> ITGRPEWIWLALGTALMGLGTLYFLVKGMGVSDPDAKKFYAITTLVPAIAFTMYLSMLLGYGLTMVPF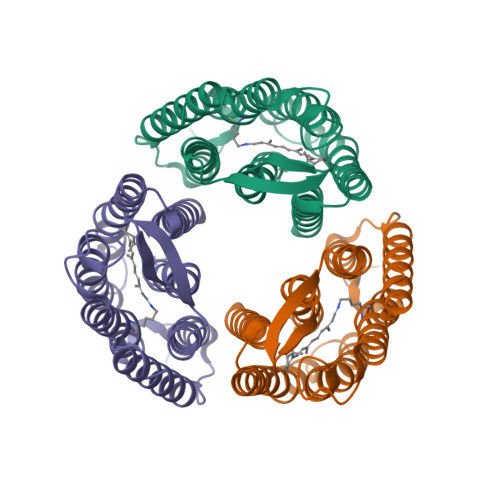GGEQNPIYWARYADWLFTTPLLLLDLALLVDADQGTILALVGADGIMIGTGLVGALTKVYSYRFVWWAISTAAMLYILYVLFFGFTSKAESMRPEVASTFKVLRNVTVVLWSAYPVVWLIGSEGAGIVPLNIETLLFMVLDVSAKVGFGLILLRSRAIFGEAE> GSHMEHVAFGSEDIENTLAKMDDGQLDGLAFGAIQLDGDGNILQYNAAEGDITGRDPKQVIGKNFFKDVAPCTDSPEFYGKFKEGVA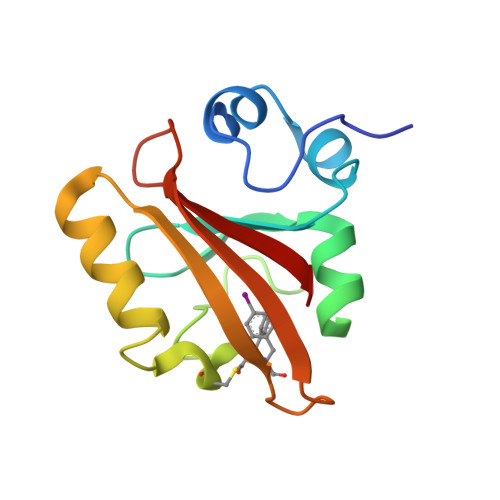SGNLNTMFEYTFDYQMTPTKVKVHMKKALSGDSYWVFVKRV> STGITYDEDRKTQLIAQYESVREVVNAEAKNVHVNENASKILLLVVSKLKPASDIQILYDHGVREFGENYVQELIEKAKLLPDDIKWHFIGGLQTNKCKDLAKVPNLYSVETIDSLKKAKKLNESRAKFQPDCNPILCNVQINTSHEDQKSGLNNEAEIFEVIDFFLSEECKYIKLNGLMTIGSWNVSHEDSKENRDFATLVEWKKKIDAKFGTSLKLSM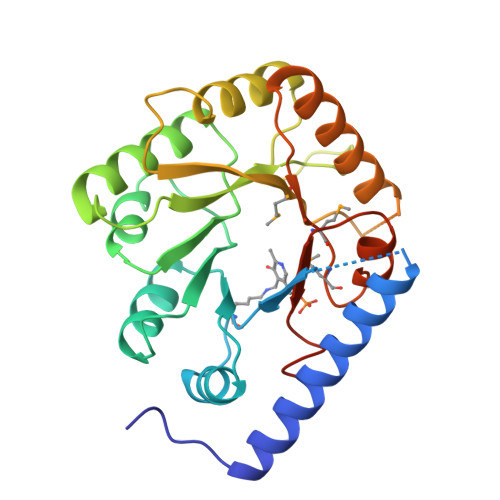GMSADFREAIRQGTAEVRIGTDIFGARPPKNEARII>[2x]GPLGSMKTVFSPLHSRRHVKTELDGGLLIEPHEKPSRAETILARVKDQALGEILEPEEFGLGPVKRVHTADYVSFLETCWDEWVAAGKRGEAIPTFWVGRGMRARLPKDIDGRLGYYSLGADTSISDGTWEAARASANVALTAQKLVAEGERAAFALCRPPGHHAHADVFGGYCFFNNAAIAAQAFRDQGYGKVAVLDVDFHHGNGTQA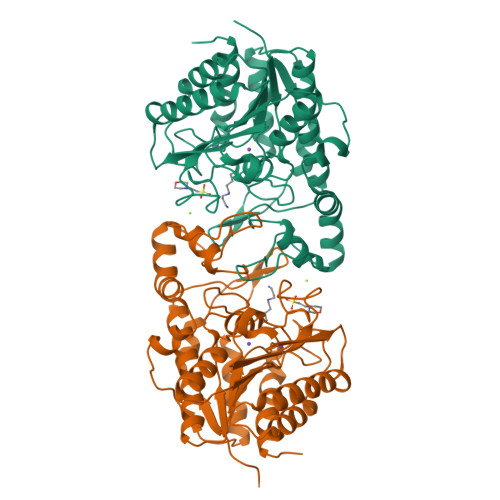IFYDRSDVLTISLHGDPDLVFPHFLGFEDETGEGDGEAYNLNIVFPPDTPFSIWSQGLEKACERIRTFAPDALVVALGVDTFEEDPISFFKLTSGDYLKLGKRLEQLGLPTVFTMEGGYDVDAIGVNAVNVMQGFEGKS> HMDKLRVLYDEFVTISKDNLERETGLSASDVDMDFDLNIFMTLVPVLAAAVCAITPTIEDDKIVTMMKYCSYQSFSFWFLKSGAVVKSVYNKL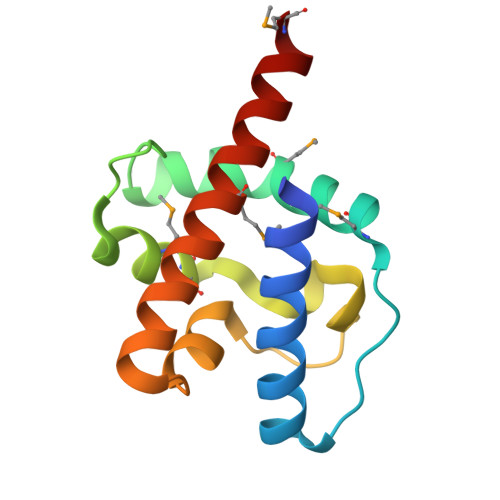DYVKKEKFVATFRDMLLNVQTLISLNSMY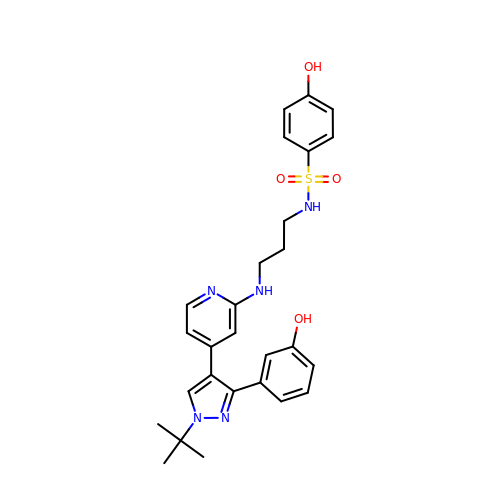N-[3-({(4P)-4-[(3M)-1-tert-butyl-3-(3-hydroxyphenyl)-1H-pyrazol-4-yl]pyridin-2-yl}amino)propyl]-4-hydroxybenzene-1-sulfonamide | C27 H31 N5 O4 S | DXOOEWGOXWQIJI-UHFFFAOYSA-N> LAGVKKDIEKLYEAVPQLSNVFKIEDKIGEGTFSSVYLATAQLQVGPEEKIALKHLIPTSHPIRIAAELQCLTVAGGQDNVMGVKYCFRKNDHVVIAMPYLEHESFLDILNSLSFQEVREYMLNLFKALKRIHQFGIVHRDVKPSNFLYNRRLKKYALVDFGLAQGTHDTKIELLKFVQSEAQQERCSQNKPASLTCDCYATDKVCSICLSRRQQVAPRAGTPGFRAPEVLTKCPNQTTAIDMWSAGVIFLSLLSGRYPFYKASDDLTALAQIMTIRGSRETIQAAKTFGKSILCSKEVPAQDLRKLCERLRGAGAGGWNEVPDEAYDLLDKLLDLNPASRITAEEALLHPFFKDMSL;> GPGTRTGRLKKPFVKVEDMSQLYRPFYLQLTNMPFINYSIQKPCSPFDVDKPSSMQKQTQVKLRIQTDGDKYGGTSIQLQLKEKKKKGYCECCLQKYE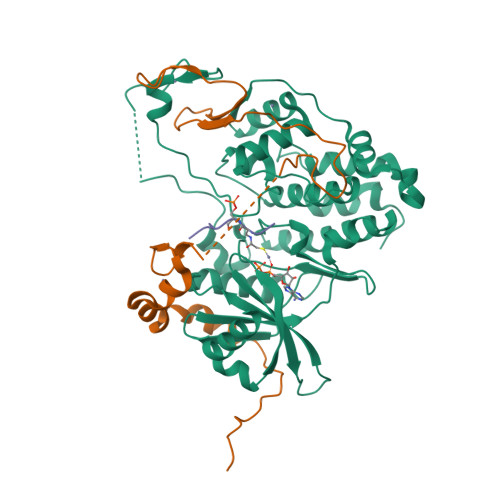DLETHLLSEQHRNFAQSNQYQVVDDIVSKLVFDFVEYEKDTPKKKR;> RRTDALTASPGRDLP>MSISISYSTTYSGWTVADYLADWSAYFGDVNHRPGQVVDGSNTGGFNPGPFDGSQYALKSTASDAAFIAGGDLHYTLFSNPSHTLWGKLDSIALGDTLTGGASSGGYALDSQEVSFSNLGLDSPIAQGRDGTVHKVVYGLMSGDSSALQGQIDALLKAVDPSLSINSTFDQLAAAGVA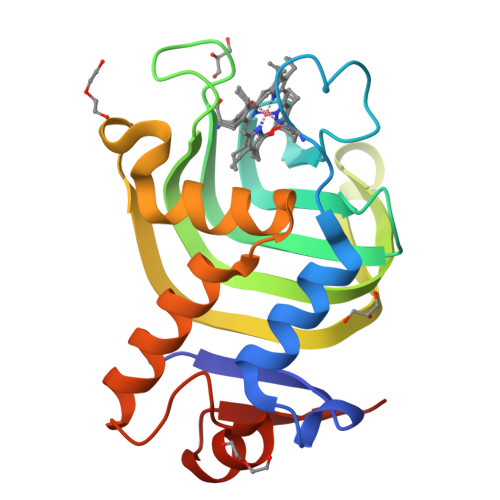HATPAA[2x]> MSAYRHAVERIDSSDLACGVVLHSAPGYPAFPVRLATEIFQRALARLPGDGPVTLWDPCCGSGYLLTVLGLLHRRSLRQ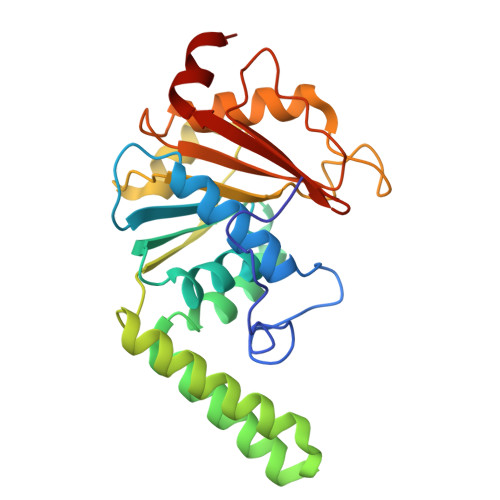VIASDVDPAPLELAAKNLALLSPAGLTARELERREQSERFGKPSYLEAAQAARRLRERLTAEGGALPCAIRTADVFDPRALSAVLAGSAPDVVLTDLPYGERTHWEGQVPAQPVAGLLRSLASALPAHAVIAVTDRSRKIPVAPVKALERLKIGTRSAVLVRAADVLEAGP>[2x]KAFKAQAKEAQQLRERAYLD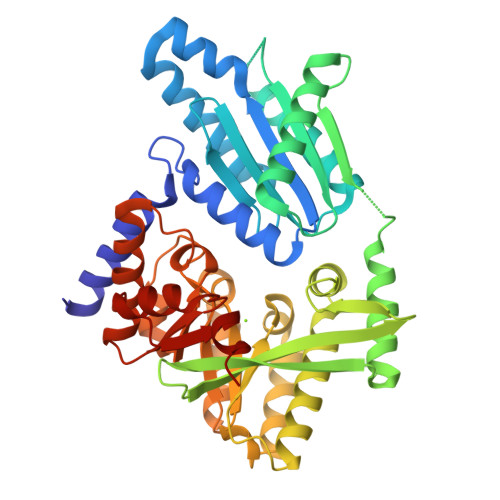PVSHLGNRAYYMSQLSGWLSESGIGGVAILQAEFIKELYEEKGYEAGDGMVRELADRLKNSITIKDISIARISTYEFGIIMPNMDETELKIVAESIITCVDDINPDPTGMAKANLSLGVVSNKRQSSTTTLLSLLDNALAKAKSNPELNYGFISSDTDKIILGKQQWKTLVEEAIHNDWFTFRYQAANSSWGKTFHREVFSAFEKDGVRYTANQFLFALEQLNASHIFDQYVIERVIQQLEKGELTDPLAINIAQGSISQPSFIRWISQTLSKHLSVANLLHFEIPEGCFVNEPHYTALFCNAVRNAGADFGVDNYGRNFQSLDYINEFRPKYVKLDYLFTHHLDDERQKFTLTSISRTAHNLGITTIASRVETQTQLDFLSEHFIEVFQGFIVDKAA> MKSVITTTISAADAAGRYPSTS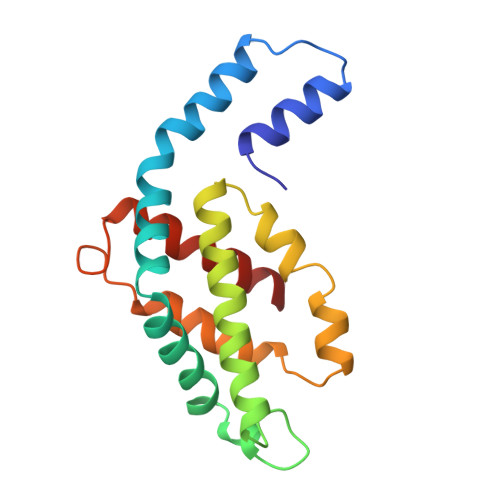DLQSVQGNIQRAAARLEAAEKLGSNHEAVVKEAGDACFSKYGYNKNPGEAGENQEKINKCYRDIDHYMRLINYTLVVGGTGPLDEWGIAGAREVYRTLNLPSAAYIAAFVFTRDRLCIPRDMSAQAGVEFCTALDYLINSLS> MSLRSKRVLVVEDNPDDIALIRRVLDRKDIHCQLEFVDNGAKALYQVQQAKYDLIILDIGLPIANGFEVMS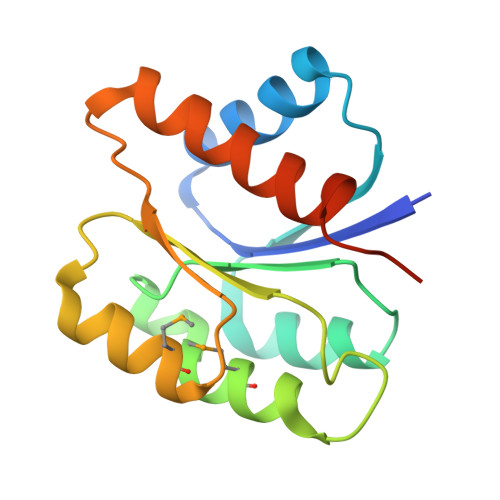AVRKPGANQHTPIVILTDNVSDDRAKQCMAAGASSVVDKSSNNVTDFYGRIYAIFSYWLTVNHCQEGHHHHHH Two racemic crystal structures of the DNA sequence d(CCCGGG) are described which were found to fold into A-form DNA. This form differs from the Z-form DNA conformation adopted by the chiral equivalent in the solid state, suggesting that the use of racemates may also favour the emergence of new conformations. Importantly, the racemic mixture forms interactions in the solid state that differ from the chiral equivalent (including the formation of racemic pseudo-helices), suggesting that the use of racemic DNA mixtures could provide new possibilities for the design of precise self-assembled nanomaterials and nanostructures.

We next turned to a sparse-matrix crystallization screening approach, which successfully identified two related conditions suitable for crystal growth. X-ray diffraction analyses of the two crystal forms indicated that the crystals belonged to the achiral space groups and P21/n, in line with previous findings describing the tendency of racemic DNA mixtures to form racemic crystals rather than conglomerates. Both crystal structures were solved by molecular replacement, with the resulting refined electron-density maps being of sufficiently high quality to allow the chirality of the DNA strands to be unambiguously determined. Analysis of the duplex geometry reveals parameters that are all in line with expectations for A-DNA, namely a rise per residue of ∼2.8–3.0 Å, a base-pair inclination of ∼9–13° and a preference for C3′-endo sugar puckers. To our knowledge, this is the first report of a racemic crystal structure of A-form DNA. The racemic A-form duplex crystal structures that we report here therefore add to the array of conformations adopted by this DNA sequence, providing further evidence of the considerable structural polymorphism of this motif. Perhaps paradoxically, despite this apparent structural polymorphism, the five independent A-type duplexes present within these two crystal structures reveal a remarkable degree of structural similarity, as indicated by structural alignments, despite the differences in space group and crystal packing. Heterochiral pseudo-continuous helices are helices in which d-DNA duplexes and l-DNA duplexes stack end-to-end in an alternating manner, with an inversion of the helix handedness at every helix–helix contact. Thus, the racemic d/l-d(CCCGGG) sequence studied here reveals packing interactions that have not previously been observed, suggesting that racemic mixtures of DNA sequences may generate assemblies and higher-order structures that are not accessible to equivalent enantiopure systems.

>CCCGGG[6x]>MSVLYTSYTKPGNWSAVDRSAWSVSCSNVYADDDAKYGAHLAIDGEINTTWFTWGVANAGECWWNTVLDRPVTLTGFSVTKQSAYGSGYNLRSAEIKVRKEGETEWVTYPRVLTFRNFKGADPQYAAIEPPIPNVKEFRINCLTPDN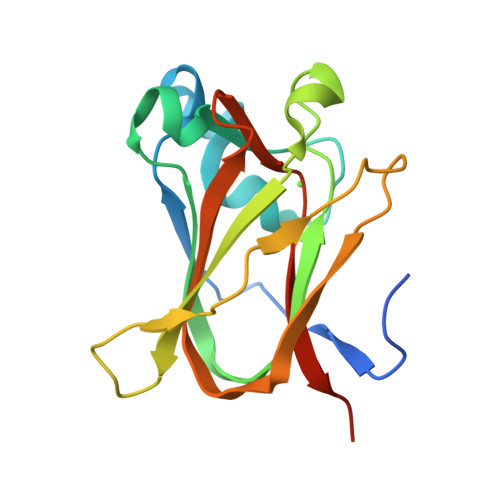YTGFAEINLYEKQLEHHHHHH[2x]Human factor D (FD) is a self-inhibited thrombin-like serine proteinase that is critical for amplification of the complement immune response. FD is a single-domain serine protease that has a unique physiological substrate. It converts the surface-bound alternative pathway pro-convertase C3bB into the active convertase C3bBb. A salt bridge between Arg202 (Arg218) on the self-inhibitory loop and Asp177 (Asp189) locks the S1 pocket and rigidifies the exosite.

The R202A (R218A) mutation disrupts a crucial interaction responsible for maintaining the self-inhibited state of FD. The previously reported crystal structure of FD R202A determined at 2.8 Å resolution showed the catalytic site in an active configuration with residual density indicating the presence of disorder, which could not be modelled. In addition, these data yielded weak electron density for a number of surface-exposed loops, suggesting high mobility and/or multiple conformations for these regions. The new map allowed a more detailed interpretation of the active site, showing multiple conformations that indicate the coexistence of both active and inactive configurations. Despite the overall improvement in electron density, however, the surface-exposed regions corresponding to the exosite loops remained poorly defined, with only few interpretable side chains. The R202A FD variant has enhanced activity towards artificial peptides and simultaneously displays active and inactive conformations of the active site. Partially active conformations of the catalytic site in FD R202A (R218A) versus completely inactive conformations for the wild type are consistent with the observed increase in the catalytic activity of FD R202A (R218A) towards artificial peptide substrates. Biophysical analyses using thermal shift assays and circular-dichroism spectroscopy showed very similar results for wild-type and R202A (R218A) FD.

>[2x]ILGGREAEAHARPYMASVQLNGAHLCGGVLVAEQWVLSAAHCLEDAADGKVQVLLGAHSLSQPEPSKRLYDVLRAVPHPDSQPDTIDHDLLLLQLSEKATLGPAVRPLPWQRVDRDVAPGTLCDVAGWGIVNHAGRRPDSLQHVLLPVLDRATCNRRTHHDGAITERLMCAESNRRDSCKGDSGGPLVCGGVLEGVVTSGSAVCGNRKKPGIYTRVASYAAWIDSVLA>MAHHHHHHVGTFENITAAPADPILGLADLFRADERPGKINLGIGVYKDETGKTPVLTSVKKAEQYLLENETTKNYLGIDGIPEFGRCTQELLFGKGSALINDKRARTAQTPGGTGALRVAADFLAKNTSVKRVWVSNPSWPNHKSVFNSAGLEVREYAYYDAENHTLDFDALINSLNEAQAGDVVLFHGCCHNPTGIDPTLEQWQTLAQLSVEKGWLPLFDFAYQGFARGLEEDAEGLRAFAAMHKELIVASSYSKNFGLYNERVGACTLVAADSETVDRAFSQMKAAIRANYSNPPAHGASVVATILSNDALRAIWEQELTDMRQRIQRMRQLFVNTLQEKGANRDFSFIIKQNGMFSFSGLTKEQVLRLREEFGVYAVASGRVNV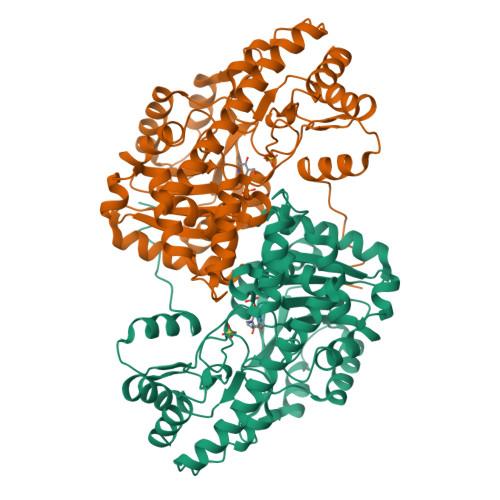AGMTPDNMAPLCEAIVAVL[2x]> YDRAITVFSPD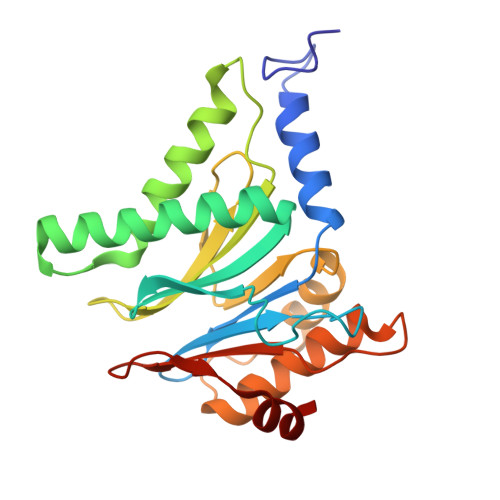GRLFQVEYAREAVKKGSTALGMKFANGVLLISDKKVRSRLIEQNSIEAIQLIDDYVAAVTSGLVADARVLVDFARISAQQEKVTYGSLVNIENLVKRVADQMQQYTQYGGVRPYGVSLIFAGIDQIGPRLFDCDPAGTINEYKATAIGSGKDAVVSFLEREYKENLPEKEAVTLGIKALKSSLEEGEELKAPEIASITVGNKYRIYDQEEVKKFL>MRENNSGEKTRVLVVGGTGTMGRRIVRACLAEGHETYVLQQPETRVDIEKVQLLYSYKRLGARLIEASFSDHQSLVSAVKQVDIVVAAMSGVHFRSHSILVQLKLVEAIKEAGNIKRFLPSEFGMDPSRMGHAMPPGRETFDQKLEVRNAIEAAGIPHTYVVGACFAAYFAGNLSQMGTLIPPKKKVNIYGDGNVKVVYVDEDDIAEYTAKTLDDPRTINKTVYVRPTENVLTQMELVQIWEKLTGKELEKTNISANDF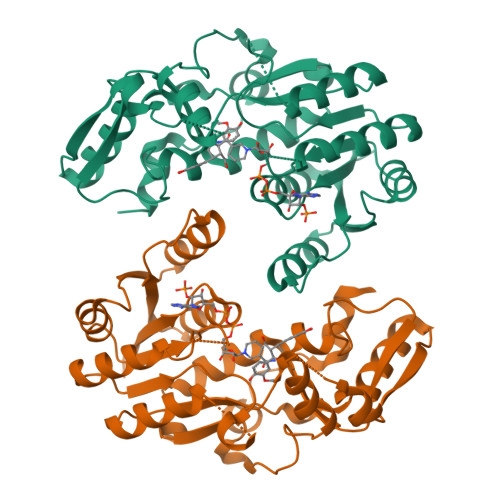LADIEDKEIPHQAGLGHFYHIFYEGCLTDHEVGDDEEASKLYPDVKYTRMDEYLKIFL[6x]>[4x]KIFKPEELRQALMPTLEALYRQDPESLPFRQP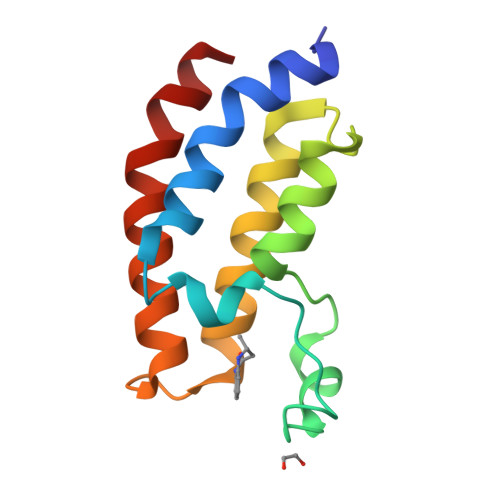VDPQLLGIPDYFDIVKNPMDLSTIKRKLDTGQYQEPWQYVDDVWLMFNNAWLYNRKTSRVYKFCSKLAEVFEQEIDPVMQSL> DRITATAYNEKRRNGELGEHILLDTREKEHFSFGSIPGAVNV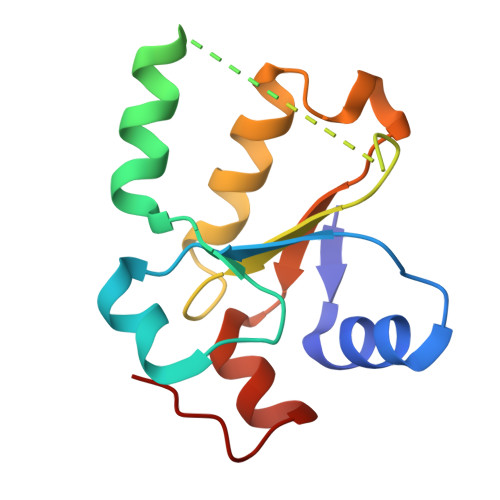PFSKFLVKASSIKREGNSPAELLPMQPASDEAPIVVVCRRGQDSQEVVEKLKELGLDNGGKRKIMDIVGGMKAWRDEVDPDFPFI5-(3-chlorophenyl)-6-(3-phenoxypropyl)pyrimidine-2,4-diamine | 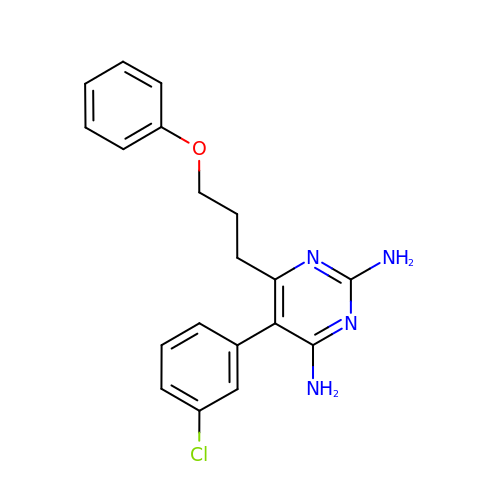C19 H19 Cl N4 O | XMRJZVVWOPBOKP-UHFFFAOYSA-N The HH ligand is secreted into the extracellular space by a cell surface protein named Dispatched-1 (DISP1). DISP1 is a well-studied isoform that contains 1,524 amino acid residues, including a ∼170-residue N-terminal intracellular domain (NTD), 12 transmembrane helices (TMs), two extracellular domains (ECDs), and a ∼300-residue C-terminal intracellular domain (CTD). As a member of the resistance–nodulation–division (RND) transporters, DISP1 shares a similar topology with PTCH1, NPC1, and bacterial efflux transporters such as AcrB. TMs 2-6 of DISP1 form the sterol-sensing domain (SSD), which is widely conserved among polytopic membrane proteins involved in cholesterol metabolism and transport (e.g., PTCH1 and NPC1).

The construct referred to as DISP1* with an N-terminal truncation (Δ1-171) and a C-terminal truncation (Δ1249-1524) yielded high expression in HEK cells with ideal behavior in a detergent solution. The structure of DISP1* was determined at 4.5-Å resolution; because of the higher local resolution, the TMs are well modeled and most aromatic residues could be assigned. Because the DISP1* protein appears as two bands on an SDS–PAGE and the loop region 253–292 is invisible in the cryo-EM map, we speculated that the recombinant DISP1* was cleaved by Furin, which is consistent with a previous study showing that Furin-mediated cleavage is required for DISP1 maturation and localization. The ECDs of PTCH1 and NPC1 twist together to create an intermolecular tunnel for cholesterol transport; in contrast, ECD-I of DISP1* is shifted from ECD-II by more than 15 Å, which is not observed in either NPC1 or PTCH1, leading to an open conformation of the two ECDs in DISP1*. On the other hand, the loop between residues 253–292, which is absent in both PTCH1 and NPC1, is disordered in the map, indicating that the flexibility of this large loop permits it to be accessible to Furin and the cleavage by Furin may release this internal loop to facilitate the endosomal trafficking of DISP1. An internal C2 symmetry is found in the TMs of DISP1*. Similar to the sterol-like molecules found in the TMs of PTCH1, five sterol-like molecules are observed in the TMs of DISP1. We tentatively assign these molecules as cholesteryl hemisuccinate (CHS) based on the density shapes and the hydrophobic environment that is created by potential binding residues. One is found in the sterol-binding pocket of the SSD (site 1), and two are found near the N terminus of TM12 (site 2). There are two novel sterol-binding sites in DISP1*: One is located in the pocket created by TMs 7-10 (site 3) in a position that is symmetrically related to the sterol in the SSD.

> MAWSHPQFEKSRPFKLPKSYAALIADWPVVVLGMCTMFIVVCALVGVLVPELPDFSDPLLGFEPRGTAIGQRLVTWNNMVKNTGYKATLANYPFKYADEQAKSHRDDRWSDDHYEREKREVDWNFHKDSFFCDVPSDRYSRVVFTSSGGETLWNLPAIKSMCNVDNSRIRSHPQFGDLCQRTTAASCCPSWTLGNYIAILNNRSSCQKIVERDVSHTLKLLRTCAKHYQNGTLGPDCWDMAARRKDQLKCTNVPRKCTKYNAVYQILHYLVDKDFMTPKTADYATPALKYSMLFSPTEKGESMMNIYLDNFENWNSSDGVTTITGIEFGIKHSLFQDYLLMDTVYPAIAIVIVLLVMCVYTKSMFITLMTMFAIISSLIVSYFLYRVVFHFEFFPFMNLTALIILVGIGADDAFVLCDVWNYTKFDKPHAETSETVSITLQHAALSMFVTSFTTAAAFYANYVSNITAIRCFGVYAGTAILVNYVLMVTWLPAVVVLHERYLLNIFTCFKKPQQQIYDNKSCWTVACQKCHKVLFAISEASRIFFEKVLPCIVIKFRYLWLFWFLALTVGGAYIVCINPKMKLPSLELSEFQVFRSSHPFERYDAEYKKLFMFERVHHGEELHMPITVIWGVSPEDNGNPLNPKSKGKLTLDSSFNIASPASQAWILHFCQKLRNQTFFYQTDEQDFTSCFIETFKQWMENQDCDEPALYPCCSHWSFPYKQEIFELCIKRAIMELERSTGYHLDSKTPGPRFDINDTIRAVVLEFQSTYLFTLAYEKMHQFYKEVDSWISSELSSAPEGLSNGWFVSNLEFYDLQDSLSDGTLIAMGLSVAVAFSVMLLTTWNIIISLYAIISIAGTIFVTVGSLVLLGWELNVLESVTISVAVGLSVDFAVHYGVAYRLAPDPDREGKVIFSLSRVGSAMAMAALTTFVAGAMMMPSTVLAYTQLGTFMMLIMCISWAFATFFFQCMCRCLGPQGTCGQIPLPKKLQCSAFSHALSTSPSDKGQSKTHTINAYHLDPRGPKSELEHEFYELEPLASHSCTAPEKTTYEETHICSEFFNSQAKNLGMPVHAAYNSELSKSTESDAGSDYKDDDDK>[2x]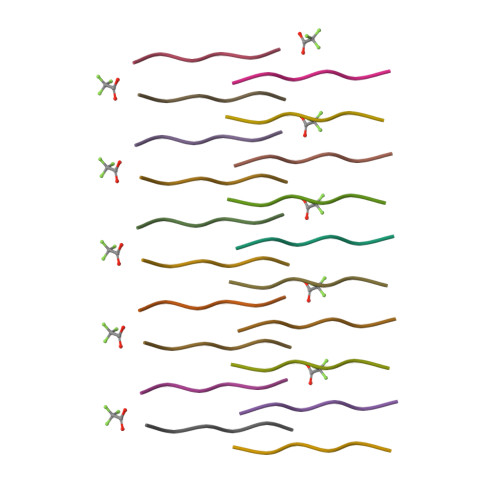FGTGFG> AEHIVEMRNKDD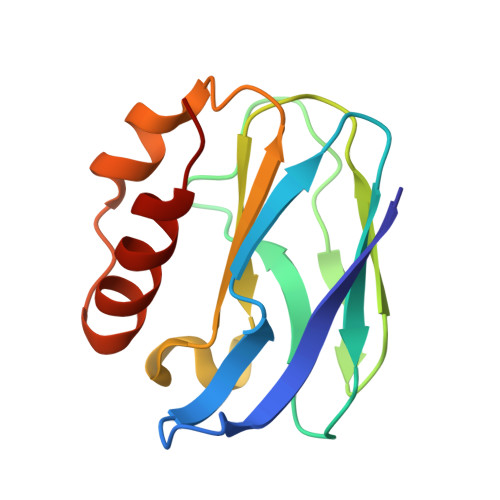AGNTMVFQPGFVKVEAGDTVKFVPTDKSHNAESVREVWPEGVAPVKGGFSKEVVFNAEKEGLYVLKCAPHYGMGMVVLVQVGKPVNLDQIKEYKATGLAKKRLDGEIAKVVQ> V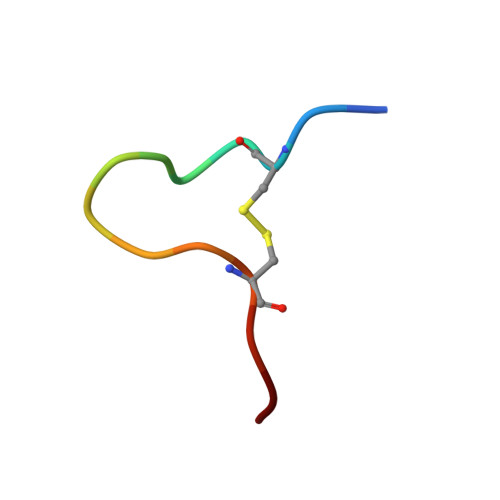PCPYLPLWNCAGK> MVEQILAEFQLQEEDLKKVMRRMQKEMDRGLRLETHEEASVKMLPTYVRSTPEGSEVGDFLSLDLGGTNFRVMLVKVGEGEEGQWSVKTKHQMYSIPEDAMTGTAEMLFDYISECISDFLDKHQMKHKKLPLGFTFSFPVRHEDIDKGILLNWTKGFKASGAEGNNVVGLLRDAIKRRGDFEMDVVAMVNDTVATMISCYYEDHQCEVGMIVGTGCNACYMEEMQNVELVEGDEGRMCVNTEWGAFGDSGELDEFLLEYDRLVDESSANPGQQLYEKLIGGKYMGELVRLVLLRLVDENLLFHGEASEQLRTRGAFETRFVSQVESDTGDRKQIYNILSTLGLRPSTTDCDIVRRACESVSTRAAHMCSAGLAGVINRMRESRSEDVMRITVGVDGSVYKLHPSFKERFHASVRRLTPSCEITFIESEEGSGRGAALVS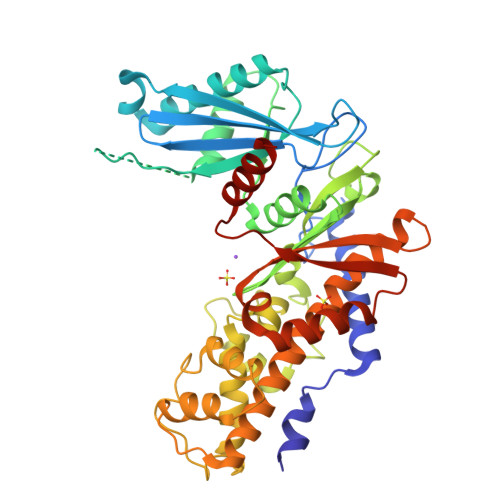AVACKKACMLGQ> IVGGTASVRGEWPWQVTLHTTSPTQRHLCGGSIIGNQWILTAAHCFYGVESPKILRVYSGILNQAEIKEDTSFFGVQEIIIHDQYKMAESGYDIALLKLETTVNYADSQRPISLPSKGDRNVIYTDCWVTGWGYRKLRDKIQNTLQKAKIPLVTNEECQKRY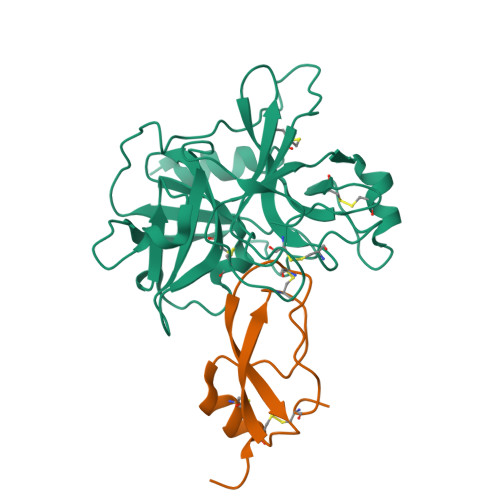RGHKITHKMICAGYREGGKDACKGDSGGPLSCKHNEVWHLVGITSWGEGCAQRERPGVYTNVVEYVDWILEKTQA;> EVCSEQAETGPCRAMISRWYFDVTEGKCAPFFYGGCGGNRNNFDTEEYCMAVCGSAI>[4x]ASKWTYFGPDGENSWSKKYPSCGGLLQSPIDLHSDILQYDASLTPLEFQGYNLSANKQFLLTNNGHSVKLNLPSDMHIQGLQSRYSATQLHLHWGNPNDPHGSEHTVSGQHFAAELHIVHYNSDLYPDASTASNKSEGLAVLAVLIEMGSFNPSYDKIFSHLQHVKYKGQEAFVPGFNIEELLPERTAEYYRYRGSLTTPPCNPTVLWTVFRNPVQISQEQLLALETALYCTHMDDPSPREMINNFRQVQKFDERLVYTSFSQ

The carbonic anhydrase (CA) family (CA, EC 4.2.1.1), consisting of twelve catalytically active human isozymes, performs the catalysis of reversible hydration of CO2 into bicarbonate and acid protons. Since it has been observed that CAIX isozyme is highly overexpressed in numerous cancers, it has been postulated that compounds inhibiting CAIX may possess the anticancer activity and may be used in tumor treatment. Here we have designed a series of compounds, methyl 5-sulfamoyl-benzoates, which bear a primary sulfonamide group, a well-known marker of CA inhibitors, and determined their affinities for all twelve CA isozymes. Eight crystal structures of CA complexes with compounds are presented in this study: 9a bound to CAI and CAII, 3b, 3d, 5b, and 9a bound to CAXII, 3b bound to CAIX and mimic-CAIX (mutant of CAII containing amino acids in the active site as in CAIX: A65S, N67Q, I91L, F130V, V134L, and L203A).

We compared the crystal structures of several compounds in two different CA isozymes. Figure 2B shows the binding mode of 3b and 3d in the active site of CAXII. The binding modes of both ligands in the active site of CAXII were the same: ortho groups were directed to the hydrophobic part of the active site, while meta substituents were orientated to the hydrophilic part. The binding affinities and enthalpy changes to CAXII were almost identical (ΔGintr = −62.3 kJ/mol, ΔHintr = −48.0 kJ/mol (3b) vs. ΔGintr = −61.1 kJ/mol, ΔHintr = −50.1 kJ/mol (3d), Figure 2B). The positions of the compounds were similar. However, the binding affinities of 3b to CAIX and CAXII differed significantly and were 150 times stronger to CAIX than CAXII (Kd_intr = 0.030 nM or ΔGintr = −62.3 kJ/mol to CAXII and Kd_intr 0.20 pM or ΔGintr = −75.0 kJ/mol to CAIX). Again, the side chains interacting with 3b in CAIX and CAXII were different. They were more hydrophobic in CAIX (A203, L135, V131, L91, and Q67) and more hydrophilic in CAXII (N204, S135, V131, T91, and K68).> QTVAIKMGADNGMLAFEPSTIEIQAGDTVQWVNNKLAPHNVVVEGQPELSH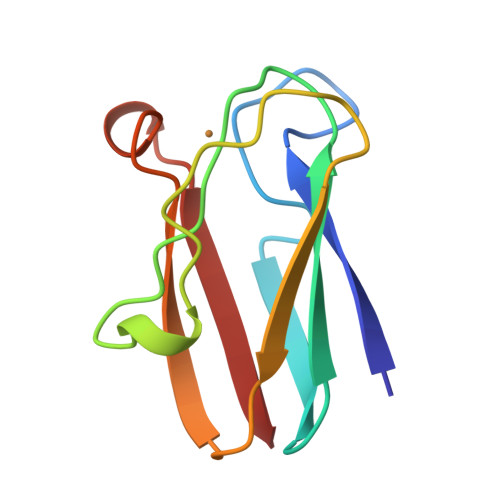KDLAFSPGETFEATFSEPGTYTYYCEPHRGAGMVGKIVVQ>[4x]MAMALALRRLSSSHRLSNRSSLKYLSSLPNPVARDIEDSRVKWTKQLNAPLEEIDPEIADIIELEKARQWKGFELIPSENFTSLSVMQAVGSVMTNKYSEGYPGARYYGGNEYIDMAERLCQKRALEAFNLDPSKWGVNVQSLSGSPANFQVYTALLKPHERIMALDLPHGGHLSHGYQTDTKKISAVSIFFETMPYRLDESTGYIDYEQMEKSAVLFRPKLIVAGASAYARVYDYARMRKVCDKQKAILLADMAHISGLVAAGVVPSPFEYADVVTTTTHKSLRGPRGAMIFFRKGLKEINKKGEEVMYDFEDKIN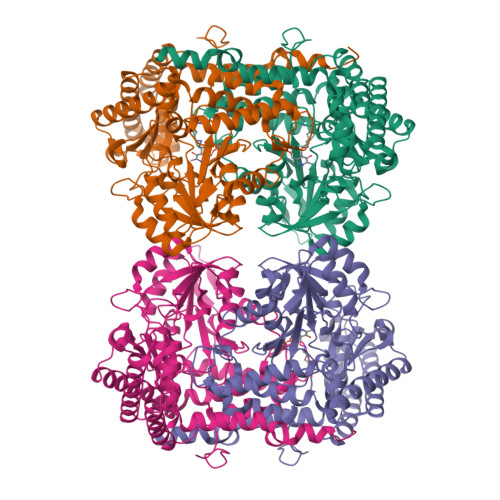QAVFPGLQGGPHNHTIAGLAVALKQATTPEYKAYQEQVLANCKRFSQSLIERGYSLVSGGTDNHLVLVNLRDKGIDGSRVEKVMELAHIAANKNTVPGDVSAMVPGGIRMGTPALTSRGFLEEDFVKVAELFDASVKLALKIKAASSGTKLKDFVATMNGDEKFQSEIKKIRGEVEEYAKQFPTIGFEKETMKYKN>[2x]MAVPETRPNHTIYINNLNEKIKKDELKKSLHAIFSRFGQILDILVSRSLKMRGQAFV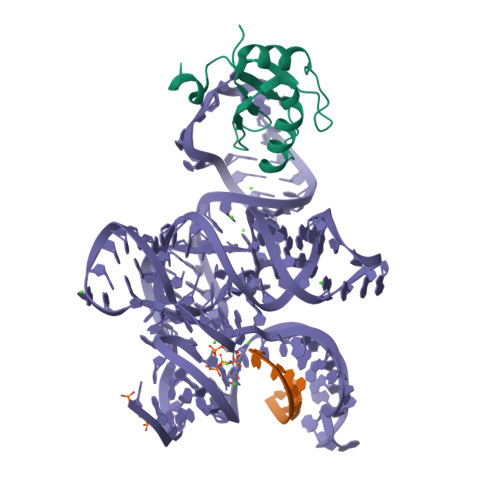IFKEVSSATNALRSMQGFPFYDKPMRIQYAKTDSDIIAKMK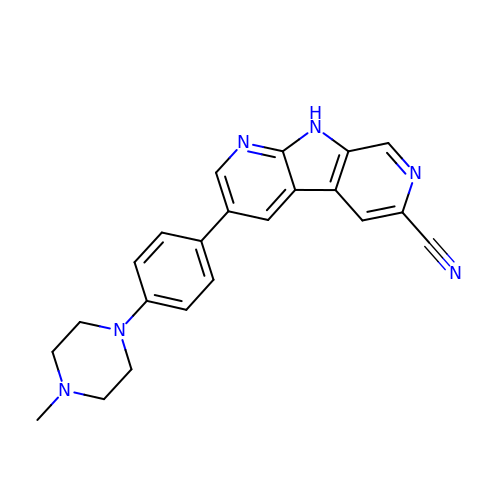3-[4-(4-methylpiperazin-1-yl)phenyl]-9H-pyrrolo[2,3-b:5,4-c']dipyridine-6-carbonitrile | C22 H20 N6 | PVRJSOWSQUNARV-UHFFFAOYSA-N>[2x]MGIQLLDKYQLQPLSLDSVPWRRQPGQQVLWIGCSDSGCDELESSGLPADEIFAYRSLGNMM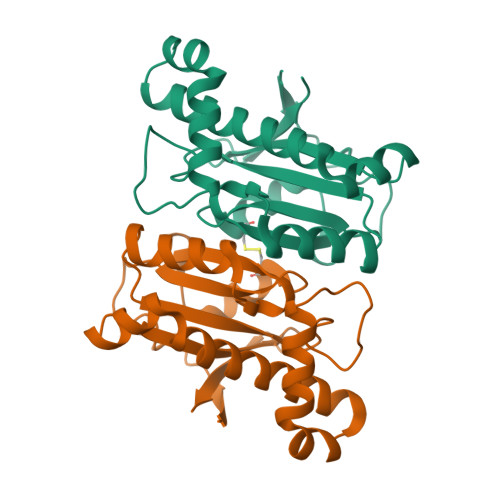VDDLSCKATLGYALDSLKIRNIVICGHYGCHIASGEVNAGLQKPWSSVLDTLRSTHRRTLDSLTGTERDRALVELNVLEQVHSLRQSAEAAEALQKQQLNIWGMVYDKATKRGYQLIEA> GMKSILEQLSSMTVVVADTGDLDSIKKFQPRDATTNPSLILAAAKNPDYVKLIDKAIESSENTLPNGFSEIELIKETVDQVSVFFGKEILKIISGRVSTEVDARLSFDTEATVKKARKLINLYKNFGIEKERILIKIAATWEGIKAAEILEKEGIKCNLTLLFNFCQAVTCANANITLISPFVGRILDWHKAKTGKTSFIGAEDPGVISVTQIYKYFKEKGFKTEVMGASFRNLDEIKELAGCDLLTIAPKFLEELKREKGVLIRKLDASTKINNSIDYKFEEKDFRLSMLEDQMASEKLSEGITGFSKAIEELEELLIERLS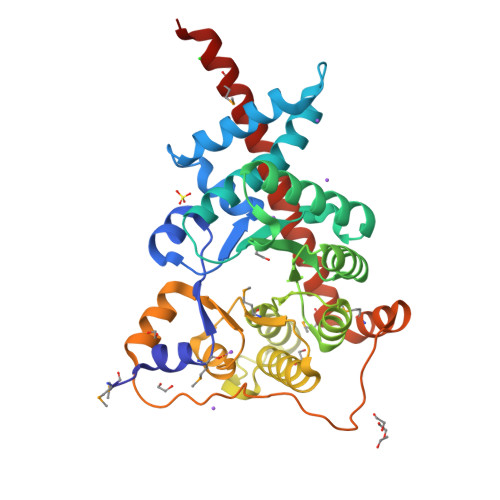EMKNHKLISAN Here we examined the factors that define the oligomeric state in a circular protein oligomer by studying the Bacillus trp RNA-binding attenuation protein (TRAP). Studies on B. subtilis have shown that when TRAP is activated by bound tryptophan, it can recognize and bind specific segments of RNA. When the tryptophan concentration is high transcription attenuation occurs as TRAP, binding to the leader RNA region of the trpEDCFBA operon transcript, induces the formation of a transcription terminator hairpin thus preventing the establishment of an antiterminator structure. When the concentration of tryptophan is limiting, TRAP is inactive, which allows transcription to proceed into the structural genes.

Unlike most other Bacillus species, the RNA leader region in the alkaliphilic bacterium B. halodurans contains 19 NAG triplets, which could potentially interact with TRAP. The oligomeric state of B. halodurans TRAP was unknown and we speculated that it might contain more than eleven subunits. In this report we show that B. halodurans TRAP forms 12-subunit assemblies, unlike the B. subtilis and B. stearothermophilus TRAP that form 11-subunit oligomers. The main chain r.m.s. difference between residues 8–70 of B. stearothermophilus TRAP 11-mer (wild type) and B. halodurans TRAP 12-mer is 0.48 Å, indicating that the 11-mer to 12-mer transition is not accompanied by significant conformational changes in the protein. The transition is achieved largely by the 2.7° rigid-body rotation of individual subunits around inter-subunit axes. The 2.7° rigid-body rotation of individual subunits is accompanied by much smaller positional adjustments in individual residues easily accommodated by the plasticity in the protein's structure. These adjustments serve to maintain the interface and its individual contacts while allowing the overall rotation of subunits with respect to each other. The 2.7° rotation of neighboring subunits with respect to each other is possible owing to a significant change in the conformation of the five C-terminal amino acids in B. halodurans TRAP. Comparison of the B. halodurans TRAP structure with the available structures of TRAP 11-mers indicated that the C-terminal segment consisting of residues 71–75 plays a critical role in selecting between 11-mer and 12-mer TRAP.

>SNFFVIKAKENGVNVFGMTRGTDTRFHHSEKLDKGEVMIAQFTEHTSAVKIRGKAIIQTSYGTLDTEKDE[3x]>QHHGVTKCN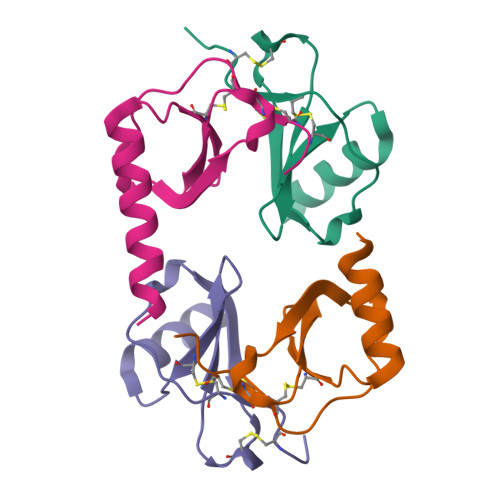ITCSKMTSKIPVALLIHYQQNQASCGKRAIILETRQHRLFCADPKEQWVKDAMQHLDRQAAALTRDG[4x]> MIVTQDKALANVFR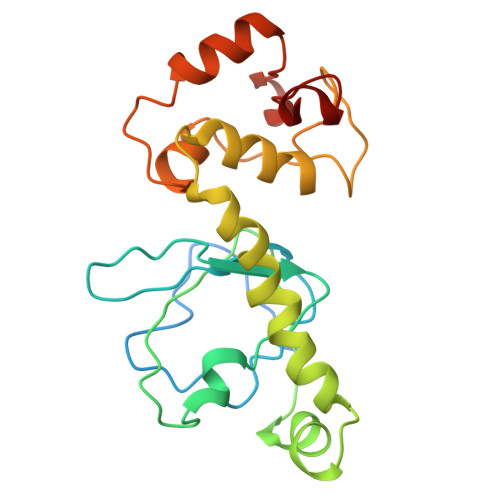QMATGAFPPVVETFERNKTIFFPGDPAERVYFLLKGAVKLSRVYEAGEEITVALLRENSVFGVLSLLTGNKSDRFYHAVAFTPVELLSAPIEQVEQALKENPELSMLMLRGLSSRILQTEMMIETLAHRDMGSRLVSFLLILCRDFGVPCADGITIDLKLSHQAIAEAIGSTRVTVTRLLGDLREKKMISIHKKKITVHKPVTLSRQFT> MDKYNNYSNVIKNKSSISPLLAAAAKIEPEITVLSSASKSNRSQYSQSLADTLLGLGYRSIFDIAKVSRQRFIKRHDESLLGNGAVIFDKAVSMANQVLQKYRKNRLEKSNSPLVPQTSSSTDASSESQTNKLPEYNQLFPEPWDNFCRPGAIEALDSPASYLLDLYKFIQSVELDGSNQARKLETRRADIPKLSLDNDALYKEVTALSIVNDVLSGSAREYIDQSGQADKAVNQILGDTHFPFTLPYSLPTQQINKGLGASNIELGTVIQRVDPQFSWNTTQEKYNQVLLAYTQLSSEQIALLSLPDVFTQNFLTQTELSAGYLSASTTEILAEKDLSRHGYIVKAADNIKGPTQLVEHSDASYDVIELTCTNQAKETITVKLRGENIITYQRTKARMVPFDNSSPFSRQLKLTFVAEDNPSLGNLDKGPYFANMDIYAAEWVRENVSSETMVSRPFLTMTYRIAIAKAGASLEELQPEADAFFINNFGLSAEDSSQLVKLVAFGDQTGSKAEEIESLLSCGENLPIVSPNVIFANPIFGSYFNDEPFPAPYHFGGVYINAHQRNAMTIIRAEGGREIQSLSNFRLERLNRFIRLQRWLDLPSHQLDLLLTSVMQADADNSQQEITEPVLKSLGLFRHLNLQYKITPEIFSSWLYQLTPFAVSGEIAFFDRIFNREQLFDQPFILDGGSFTYLDAKGSDAKSVKQLCAGLNISAVTFQFIAPLVQSALGLEAGTLVRSFEVVSSLYRLVSIPQTFGLSTEDGLILMNILTDEMGYLAKQPAFDDKQTQDKDFLSIILKMEALSAWLTKNNLTPASLALLLGVTRLAVVPTNNMVTFFKGIANGLSENVCLTTDDFQRQELEGADWWTLLSTNQVIDDMGLVLDIHPVWGKSDEEMLMEKIQSIGVSNDNNTLSIIVQILIQAKNAQENLLSQTISAEYGVERSVVPLQLRWLGSNVYSVLNQVLNNTPTDISSIVPKLSELTYSLLIYTQLINSLKLNKEFIFLRLTQPNWLGLTQPKLSTQLSLPEIYLITCYQD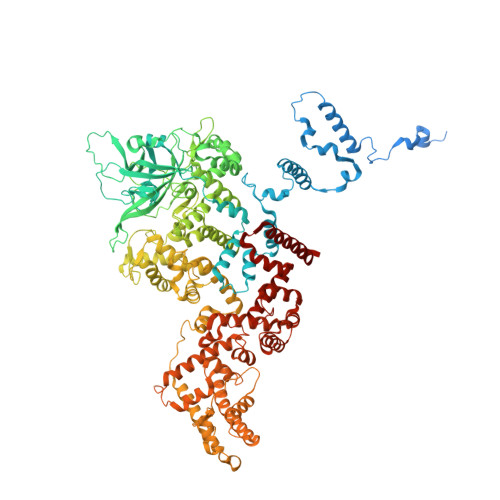WVVNANKNEDSIHEYLEFANIKKTEAEKTLVDNSEKCAELLAEILAWDAGEILKAASLLGLNPPQATNVFEIDWIRRLQTLSEKTMISTEYLWQMGDLTENSEFSLKEGVGEAVMAALKAQGDSDNV Amine transaminases (ATAs, EC 2.6.1.x) are enzymes with great potential in biocatalysis for the enantioselective synthesis of chiral primary amines from pro-chiral ketones. One of the main factors limiting the implementation of transaminases on an industrial scale for the synthesis of chiral amines is their poor storage and operational stability. In the present paper we have described and validated a possible inactivation model for the well-characterized homodimeric (S)-selective amine transaminase from Chromobacterium violaceum. Computational and experimental studies show that the stabilization role of PLP is exerted primarily at the level of the catalytic lysine K288 and secondarily at the level of the PGBC.

The cryo-protection of single holo-Cv-ATA protein crystals in the presence of the amino donor 1-(S)-phenylethylamine (20 mM) led to the conversion of PLP to PMP in cristallo without producing any visible crystal cracking (Supplementary). The final refined structure model (Supplementary) contains two homodimers per asymmetric unit, reciprocally oriented according to the same weak translational pseudo-symmetry described for the holo-form of the enzyme and each showing the same overall backbone folding. The clear discontinuity in the electron density between the cofactor ring and the K288 side chain (Supplementary) justified the modeling of the cofactor moiety as PMP in all chains with 100% occupancy. In agreement with what has been observed for other PLP-dependent enzymes, the conversion of PLP to PMP is associated with a small combined tilt and twist reorientation of the cofactor ring hinged on its pyridine nitrogen (Supplementary). The side chain of K288 was modeled with 100% occupancy in the forward conformation with only the three most terminal side chain atoms tilted away from the amino group of PMP (Supplementary). The PMP·Cv-ATA structure shows that, upon breakage of the K288-PLP Schiff base linkage, neither K288 nor the other variability regions rearrange to their apo-conformation on the seconds time scale of cryoprotection. Since the actual reaction turnover is expected to be orders of magnitude faster, it can be concluded that these structural rearrangements do not occur during the catalytic cycle and must be the outcome of a different process. The newly solved PMP·Cv-ATA crystal complex confirmed that none of the known conformational rearrangements occur on the second time scale of crystal cryoprotection and, by extension, during the much faster time scale of catalytic turnover. Recently Börner et al. reported that Cv-ATA incubation in the presence of an amine substrate results in enzyme de-stabilization and explained this observation with the possible diffusion of the non-covalently bound PMP away from the active site. This is in agreement with our model, as the conversion of PLP to PMP releases the K288 from the Schiff base constraint and enables the K288 reorientation to the backward conformation.

>[4x]HHHHHHMQKQRTTSQWRELDAAHHLHPFTDTASLNQAGARVMTRGEGVYLWDSEGNKIIDGMAGLWCVNVGYGRKDFAEAARRQMEELPFYNTFFKTTHPAVVELSSLLAEVTPAGFDRVFYTNSGSESVDTMIRMVRRYWDVQGKPEKKTLIGRWNGYHGSTIGGASLGGMKYMHEQGDLPIPGMAHIEQPWWYKHGKDMTPDEFGVVAARWLEEKILEIGADKVAAFVGEPIQGAGGVIVPPATYWPEIERICRKYDVLLVADEVICGFGRTGEWFGHQHFGFQPDLFTAAKGLSSGYLPIGAVFVGKRVAEGLIAGGDFNHGFTYSGHPVCAAVAHANVAALRDEGIVQRVKDDIGPYMQKRWRETFSRFEHVDDVRGVGMVQAFTLVKNKAKRELFPDFGEIGTLCRDIFFRNNLIMRACGDHIVSAPPLVMTRAEVDEMLAVAERCLEEFEQTLKARGLA>MALLTPDDLININMQLQKADSAVQEVTGLDIKGICKALYGTFSSSEKVGIVPVTSGNGIIGNFSASLHAITQYFGFDSFVTDMPDVSGYYEAVQNGAEIILMADDRTFLAHNLKNGKMANNQPCTGIIYAEIASRYLKADSKDVLVVGLGKVGFPGAEHLVQKDFRVYGYDADETLLERATSNLGIIPFDPANPKKFSIIFEATPCANTIPEAVLSENCVLSTPGIPCAISEELRDKYEVQLIAEPLGIGTAS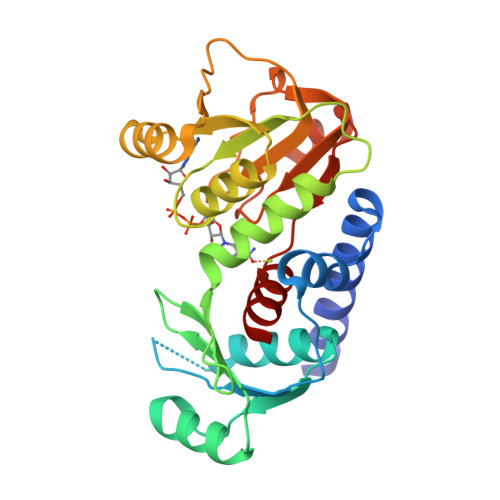MLYSVL[2x]> MSSTKRQKNRVLVKLKKRKVRKDKIEKWAELALSALGLNNVELSVYITDDQEIRELNKTYRKKDKPTDVLSFPMGEEFGGYKILGDVVISQDTAERQARELGHSLEEEVKRL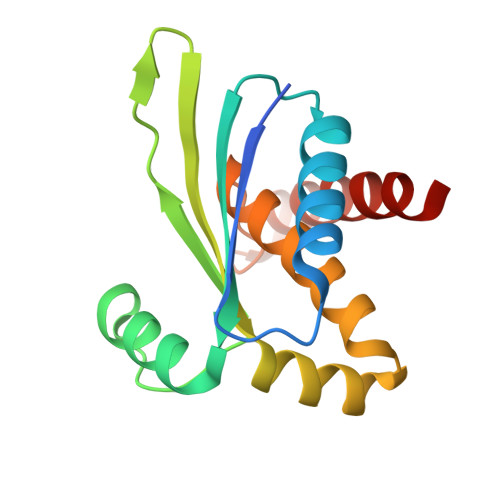IVHGIVHLLGYDHEKGGEEEKKFRELENYVLSKLSKAL The coat proteins (CPs) of single-stranded RNA bacteriophages (ssRNA phages) directly assemble around the genomic RNA (gRNA) to form a near-icosahedral capsid with a single maturation protein (Mat) that binds the gRNA and interacts with the retractile pilus during infection of the host. The canonical ssRNA phage Qβ has a genomic RNA (gRNA) of 4217 nucleotides, from the 5′ to the 3′ end, encoding the maturation protein (Mat); the major coat protein (CP); the minor capsid protein A1, which is a read-through extension caused by a leaky stop codon for the major CP; and the β-subunit of the RNA-dependent RNA replicase (Rep). Like many other viruses, the CPs of ssRNA phages can also assemble into virus-like particles (VLPs), which are not infectious. Through a native infection without engineering the amino acid sequences, we found that Qβ CP can form diverse VLP capsids, including the T = 3 icosahedral, T = 4 icosahedral, prolate, oblate, and a small prolate form elongated along the 3-fold axis.

Surprisingly, we have also observed that about 1.7% of the VLPs show a “walnut-like” prolate shape. A 3D reconstruction of these particles reveals that they are a prolate form with T = 3 and Q = 4, where T and Q describe the triangulation number of the two caps and the elongated faces, respectively. The elongated faces of the small prolate consist of two triangulation numbers, Q1 = 2 and Q2 = 3. Figure 3A shows the five forms of the VLPs from the wild-type Qβ, each containing 240, 210, 180, 150, and 132 CP copies for the T = 4, prolate, T = 3, oblate, and small prolate forms, respectively. Though all of the 5 forms contain 12 copies of the pentamers, they consist of 30, 25, 20, 15, and 12 copies of the hexamers for the T = 4, prolate, T = 3, oblate, and small prolate forms, respectively. For the prolate VLP, there are three types of hexamers. The “normal arched” type, which comes from the prolate, oblate, small prolate, and regular T = 3 capsids, has a θ angle of ~155°. Interestingly, the hexamer located on the equator of the prolate capsid has an arch angle of ~180°, which is defined as a “straight” type. The same procedure can be repeated to generate a prolate capsid from a T = 3 capsid. One can even repeatedly add hexamers in a multiplication of five in the middle of the prolate to obtain the rod-like VLP particles previously engineered.

>[21x]MAKLETVTLGNIGKDGKQTLVLNPRGVNPTNGVASLSQAGAVPALEKRVTVSVSQPSRNRKNYKVQVKIQNPTACTANGSCDPSVTRQAYADVTFSFTQYSTDEERAFVRTELAALLASPLLIDAIDQLNPAY> CW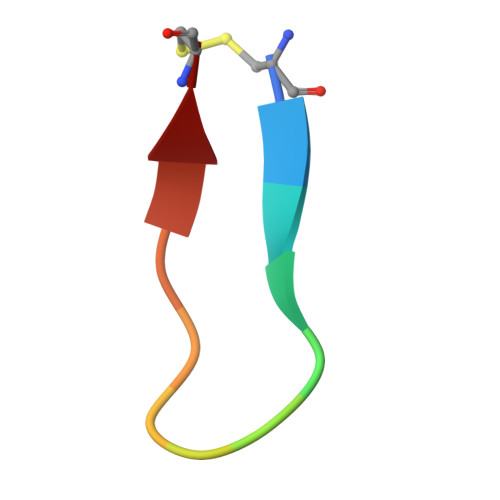TTRMSPPQQIC>[2x]HQLKLLKDDFFASDQQA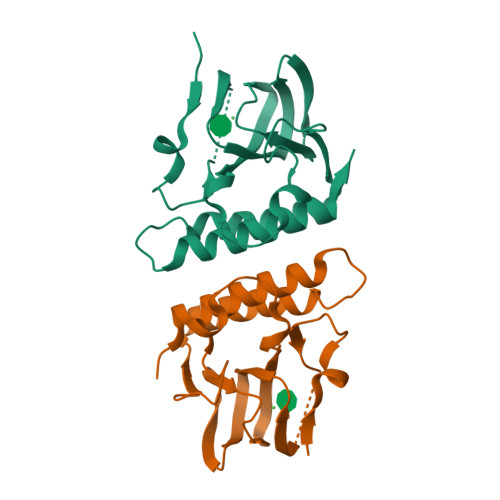VAVADRVPQDVFAEHTHDFCELVIVWRGNGLHVLNDRPYRITRGDLFYIHADDKHSYASVNDLVLQNIIYCPERLKLNLDWQGAIPGFNASAGQPHWRLGSMGMAQARQVIGQLEHESSQHVPFANEMAELLFGQLVMLLNRHRYT> QSEPELKLESVVIVSRHGVRAPTKATQLMQDVTPDAWPTWPVKLGWLTPRGGELIAYLGHYQRQRLVADGLLAKKGCPQSGQVAIIADVDERTRKTGEAFAAGLAPDCAITVHTQTDTSSPDPLFNPLKTGVCQLDNANVTDAILSRAGGSIADFTGHRQTAFRELERVLNFPQSNLCLKREKQDESCSLTQALPSELKVSADNVSLTGAVSLASMLTEIFLLQQAQGMPEPGWGRITDSHQWNTLLSLHNAQFYLLQRTPEVARSRATPLLDLIKTALTPHPPQKQAYGVTLPTSVLFIAGHDTNLANLGGALELNWTLPGQ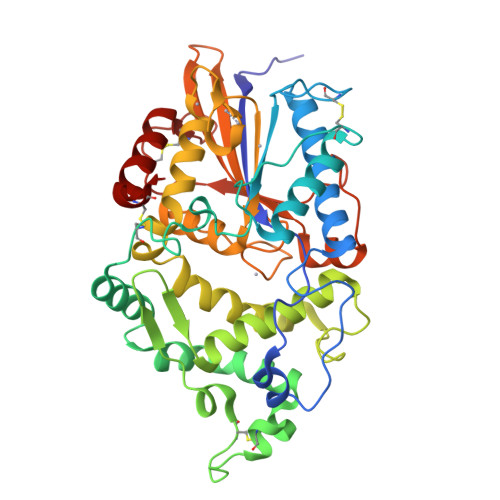PDNTPPGGELVFERWRRLSDNSQWIQVSLVFQTLQQMRDKTPLSLNTPPGEVKLTLAGCEERNAQGMCSLAGFTQIVNEARIPACSL>[2x]MANLRKVLISDSLDPCCRKILQDGGLQVVEKQNLSKEELIAELQDCEGLIVRSATKVTADVINAAEKLQVVGRAGTGVDNVDLEAATRKGILVMNTPNGNSLSAAELT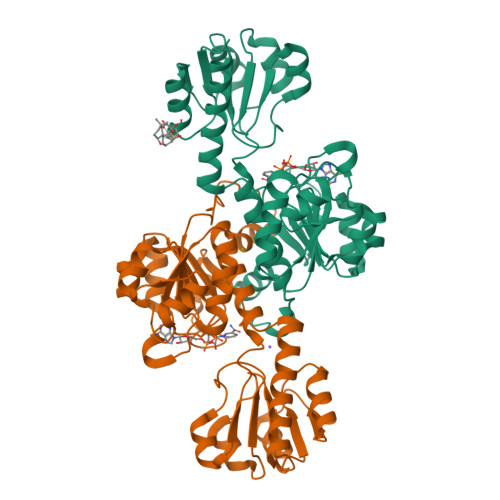CGMIMCLARQIPQATASMKDGKWERKKFMGTELNGKTLGILGLGRIGREVATRMQSFGMKTIGYDPIISPEVSASFGVQQLPLEEIWPLCDFITVHTPLLPSTTGLLNDNTFAQCKKGVRVVNCARGGIVDEGALLRALQSGQCAGAALDVFTEEPPRDRALVDHENVISCPHLGASTKEAQSRCGEEIAVQFVDMVKLEHHHHHH>[3x]MNMISRRKNAKALSGAVTALILVIASVIIALVVVGFAFGLFGAFTGQGTVTQVGTATLSAGTGTLTVTLKNTGAATQVTGAIINGNAASVSGQVTISAGQNTYSISLGGISSSTLQNLVGSTISLTLQLSNGQTVTVSAIITS

Type IV pili (T4P) represent one of the most common varieties of surface appendages in archaea. These filaments, assembled from small pilin proteins, can be many microns long and serve diverse functions, including adhesion, biofilm formation, motility, and intercellular communication. In this study, we present the high-resolution cryo-EM structures of the Saccharolobus islandicus REY15A mono-pilus and tri-pilus and demonstrate that archaeal type IV pilins can also polymerize into dramatically different filament structures.

The asymmetric unit in the tri-pilus is three subunits, each with a different orientation of the outer Ig-like domain. The inner long-helix domain exhibited a rise of 5.27 Å and a twist of 106.8°, similar but not identical to the symmetry for the mono-pilus (4.95 Å, 104.8°). In contrast, the outer domains formed trimers, breaking the symmetry of the inner domain where every subunit was equivalent, and had three times the inner symmetry with a rise of 15.8 Å and a twist of −39.6°. The final resolution of the tri-pilus reached 3.5 Å, as judged by map:map Fourier shell correlation (FSC), map:model FSC, and d9919. However, compared to the mono-pilin, the globular domain of tri-pilins undergoes a significant conformational change. Rather than projecting out from the N-terminal helix, it pivots almost 180° and bends towards the N-terminal helix. The relative orientation of the globular domain with respect to the N-terminal helix also varies across the three different subunits, A, B, and C, in the tri-pilus asymmetric unit. These different conformations are facilitated by a flexible Gly-Gln-Gly linker region situated between the two domains, and the cryo-EM densities for this linker region are clearly seen. In contrast to the mono-pilus, where inner helices are fully shielded by outer domains, portions of the inner helices in the tri-pilus become exposed to the solvent. In the tri-pilus, the outer domains trimerize to form a closely packed left-handed trimer protofilament, with minimal interactions between different turns of the protofilament. In contrast, in tri-pilus, the hydrophobic inner helices are not perfectly enveloped by the outer domains, suggesting reduced stability compared to the mono-pilus.>[20x]LDRADI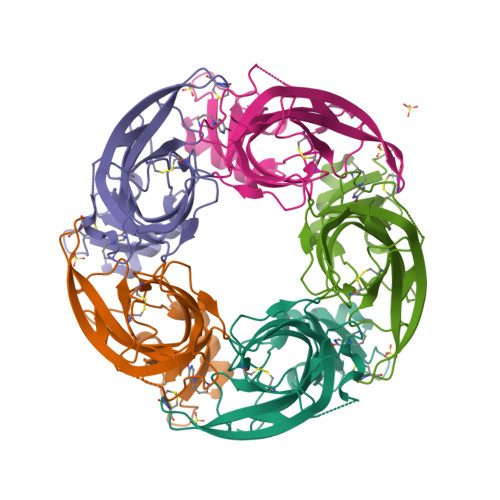LYNIRQTSRPDVIPTQRDRPVAVSVSLKFINILEVNEITNEVDVVFWQQTTWSDRTLAWNSSHSPDQVSVPISSLWVPDLAAYNAISKPEVLTPQLARVVSDGEVLYMPSIRQRFSCDVSGVDTESGATCRIKIGSWTHHSREISVDPTTENSDDSEYFSQYSRFEILDVTQKKNSVTYSCCPEAYEDVEVSLNFRKKGRSEIL(2~{S},3~{R})-3-oxidanylpyrrolidine-2-carboxylic acid | C5 H9 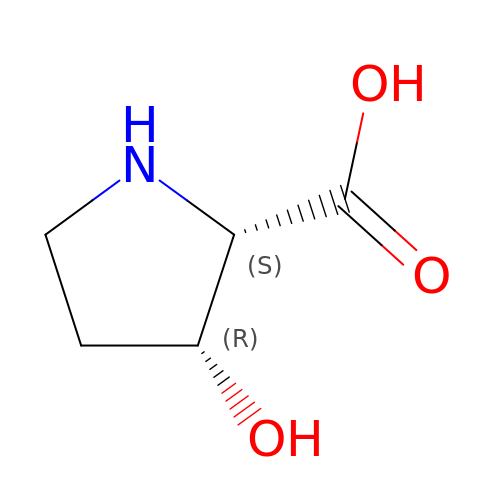N O3 | BJBUEDPLEOHJGE-DMTCNVIQSA-N> MERPESELIRQSWRVVSRSPLEHGTVLFARLFALEPSLLPLFQYNGRQFSSPEDSLSSPEFLDHIRKVMLVIDAAVTNVEDLSSLEEYLTSLGRKHRAVGVRLSSFSTVGESLLYMLEKSLGPDFTPATRTAWSRLYGAVVQAMSRGWDG

Neuroglobin (Ngb) is a member of the globin protein family that is expressed in the brain (∼1 µM) and the retina (∼100 µM) of vertebrates. It is involved in the protection of the nervous tissue from ischemic damage via a still-elusive biochemical mechanism. Notably, Ngb is also a hexacoordinate protein in the ‘deoxy’ ferrous form, with the rate-limiting step for ligand binding being the spontaneous breakage of the distal His(E7)64–heme bond.

Crystal structures of NgbCO in the ‘dark’ state (no illumination) at 40 K and of Ngb*CO obtained under continuous illumination (‘light’ state) at 15 K were determined. Upon refinement of the ‘dark’ state NgbCO, the occupancy of heme-bound CO is estimated to be about 90%. The partial CO occupancy is owing to the intrinsic instability of CO-bound Ngb crystals, which tend to dissolve upon full ligation. We therefore avoided prolonged CO soaking, with the drawback of not achieving full ligation. In this work, we only utilized crystals with at least 90% CO ligation, as assessed by its occupancy in the determined structures [Fig. 3(a)]. The presence of photolysed CO in the protein matrix, which was not visible in the Ngb*CO structure, was inferred by the full recovery of bound CO in the ‘dark’ structures collected after illumination.> GSYFSKQIIWQEVDRTKQQTSALIHNIFDSHFAAIQIHHDSNSKSEVIRDFYTDRDTDVLNFFFLSIDQSDPSHTPEFRFLTDHKGIIWDDGNAHFYGVNDLILDSLANRVSFSNNWYYINVMTSIGSRHMLVRRVPILDPSTGEVLGFSFNAVVLDNNFALMEKLKSESNVDNVVLVANSVPLANSLIGDEPYNVADVLQRKSSDKRLDKLLVIETPIVVNAVTTELCLLTVQDNQS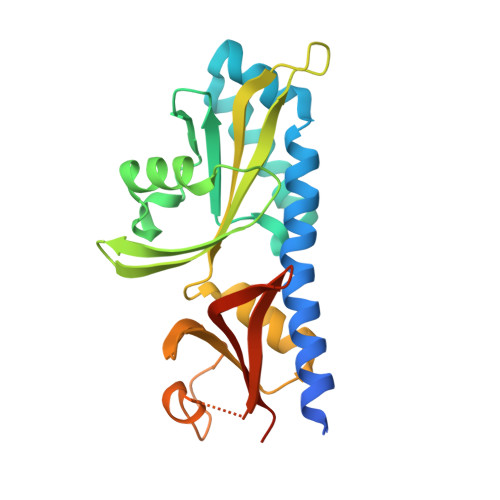VVTL> MKEKIRKKILLAPEEPGVYI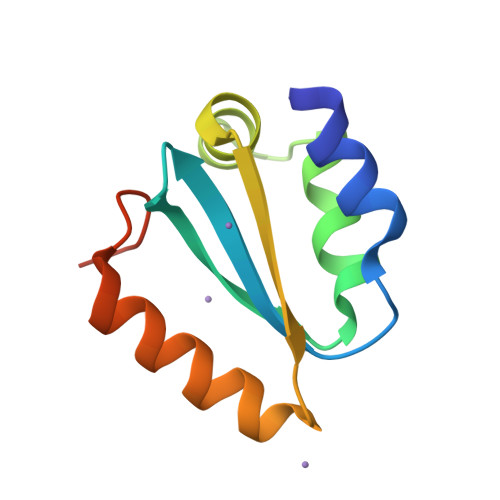FKNKGVPIYIGKAKRLSNRLRSYLNPQTEKVFRIGEEADELETIVVMNEREAFILEANLIKKYRPKYAVRLKDTDF>[2x]MRCVGVGNRDFVEGLSGATWVDVVLEHGGCVTTMAKNKPTLDIELQKTEATQLATLRKLCIEGKITNITTDSRCPTQGEAILPEEQDQNYVCKHTYVDRGWGNGCGLFGKGSLVTCAKFQCLESIEGKIVQHENLKYT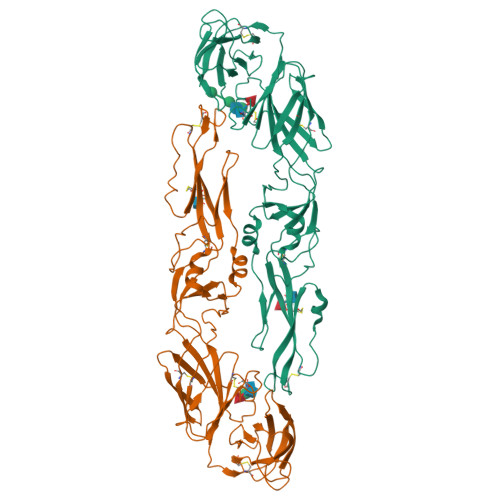VIITVHTGDQHQVGNETQGVTAEITSQASTAEAILPEYGTLGLECSPRTGLDFNEMILLTMKDKAWMVHRQWFFDLPLPWTSGATTKTPTWNRKELLVTFKNAHAKKQEVVVLGSQEGAMHTALTGATEIQTSGGTSIFAGHLKCRLKMDKLKLKGMSYAMCLNTFVLKKEVSETQHGTILIKVEYKGEDAPCKIPFSTEDGQGKAHNGRLITANPVVTKKEEPVNIEAEPPFGESNIVIGIGDKALKINWYRK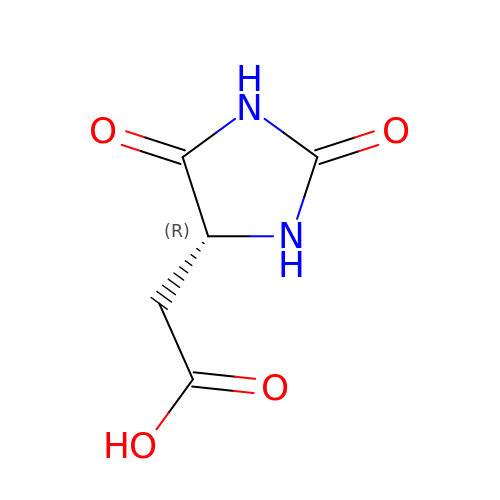[(4R)-2,5-dioxoimidazolidin-4-yl]acetic acid | C5 H6 N2 O4 | DQQLZADYSWBCOX-UWTATZPHSA-N> GSHMESGYAQNGDLEDAELDDYSFSCYSQLEVNGSQHSLTCAFEDPDVNTTNLEFEICGALVEVKCLNFRKLQEIYFIETKKFLLIGKSNICVKVGEKSLTCKKIDLTTIVKPEAPFDLSVVYREGANDFVVTFNTSHLQKKYVKVLMHDVAYRQEKDENKWTHVNLSSTKLTLLQRKLQPAAMYEIKVRSIPDHYFKGFW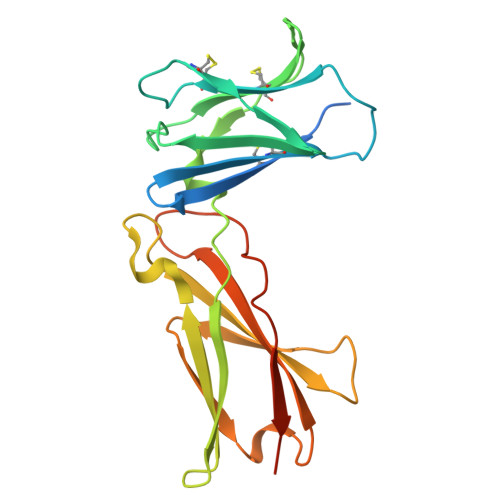SEWSPSYYFRTPEINNSSGEMD>[12x]MHH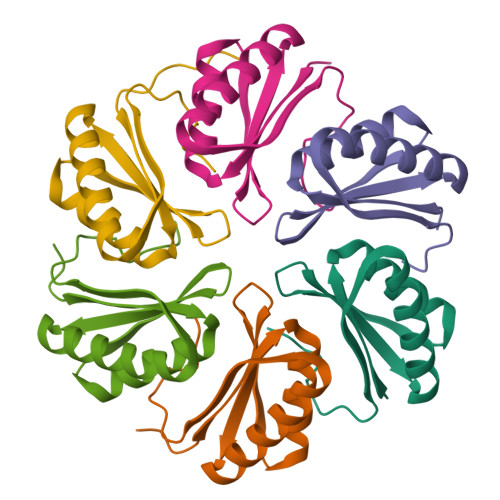HHHHMREALGLIETKGLVACIEAADAMCAAANVELIGYENVGSGLVTAMVKGDVGAVNAAVDSGVEAARRIGEVVTSRVIARPHNDIEKIASQHKA(3R,4S)-1-[(4-amino-5H-pyrrolo[3,2-d]pyrimidin-7-yl)methyl]-4-({[2-(2-hydroxyethoxy)ethyl]sulfanyl}methyl)pyrrolidin-3-ol | C16 H25 N5 O3 S | 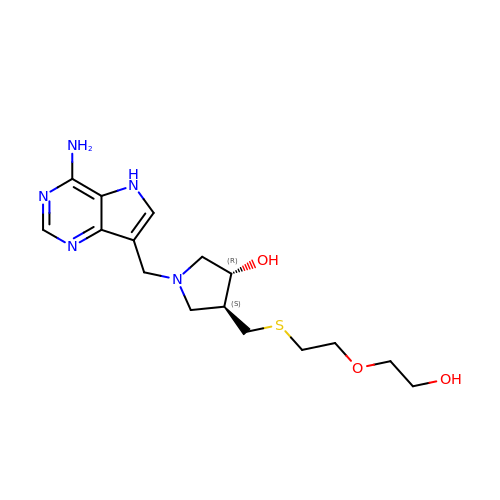OXNZLFLPEGTARO-OLZOCXBDSA-N To this end, we used the 27 nt fragment of E. coli 23 S rRNA sarcin-ricin loop (SRL) region. This sequence is known to be a robust and well-behaved crystallization scaffold that can accommodate small modifications. For the installation of 2′-OCF3, we deemed nucleotide A2670 appropriate which forms a Watson−Crick base pair with U2650 in the regular A-form double helical region of this RNA, as well as nucleotide C2667 which forms a water-mediated mismatch with U2653. The study is complemented by crystal structures of an RNA hairpin including 2′-OCF3 modifications.

We set out for the X-ray analysis of a 2′-OCF3 modified RNA. A single 2′-OCF3 adenosine exhibited only moderate attenuation of RNA double helix stability if the modification was located in the Watson–Crick base-pairing region. The 3JH1′–H2′ was clearly smaller than 1 Hz, consistent with the requirement to adopt C3′-endo conformation in an RNA double helix to avoid steric clash.

>GCUCCUAGUACGAGAGGACCGGAGUG[3x]> NPIHDRTSDYHKYLKVKQGDSDLFKLTVSDKRYIWYNPDPKERDSYECGEIVSETSDSFTFKTVDGQDRQVKKDDANQRNPIKFDGVEDMSELSYLNEPAVFHNLRVRYNQDLIYTYSGLFLVAVNPFKRIPIYTQEMVDIFKGRRRNEVAPHIFAISDVAYRSMLDDRQNQSLLITGESGAGKTENTKKVIQYLASVAGRNQANGSGVLEQQILQANPILEAFGNAKTTRNNNSSRFGKFIEIQFNSAGFISGASIQSYLLEKSRVVFQSETERNYHIFYQLLAGATAEEKKALHLAGPESFNYLNQSGCVDIKGVSDSEEFKITRQAMDIVGFSQEEQMSIFKIIAGILHLGNIKFEKGAGEGAVLKDKTALNAASTVFGVNPSVLEKALMEPRILAGRDLVAQHLNVEKSSSSRDALVKALYGRLFLWLVKKINNVLCQERKAYFIGVLDIYGFEIFKVNSFEQLCINYTNEKLQQFFNHHMFKLEQEEYLKEKINWTFIDFGLDSQATIDLIDGRQPPGILALLDEQSVFPNATDNTLITKLHSHFSKKNAKYEEPRFSKTEFGVTHYAGQVMYEIQDWLEKNKDPL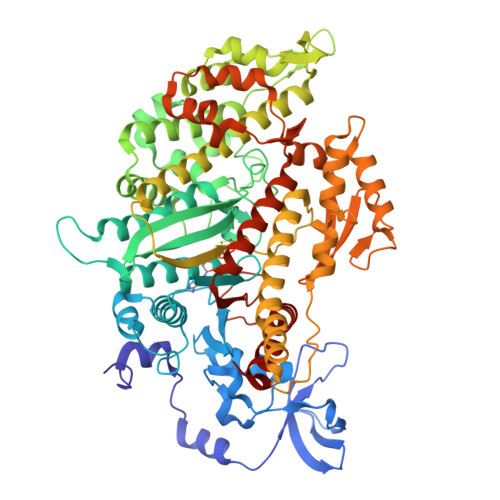QQDLELCFKDSSDNVVTKLFNDPNIASRAKKGANFITVAAQYKEQLASLMATLETTNPHFVRCIIPNNKQLPAKLEDKVVLDQLRCNGVLEGIRITRKGFP>MKKRKSSKVFKSTIAPEEKLRYIGNHKQAFDIEPLYPLALFEEFVATTGDCIIECSGKIKQDQLYPARIDLQFSDKHHFHNIHTSIDFLKRAASRTDVNLNLDILATFLAGNFDYSKVQNILAGIDLRQNLGESKLKLFIRIGDYPAKMAVAKHLCNITPESEAMLRSDT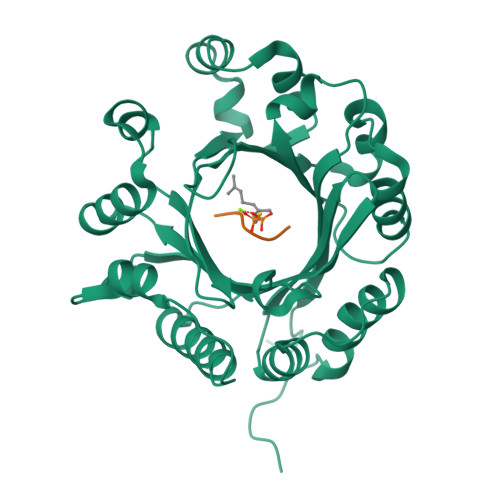LHIGFDFYLDGRSAIELYPELKKDEFNHPFIYNQLKTILSPEALKPLPLCNLFGIGLSPANEANVLYYHLENIEDFLSYFPINDTARRVHDFYLQQEGSRRMWVALSESEMKAGRINNVNLYYSKAFTSQNP[2x]> MRPPFTYATLIRWAILEAPEKQRTLNEIYHWFTRMFA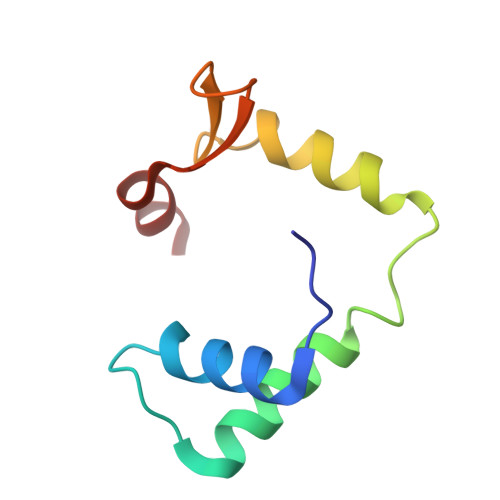FFRNHPATWKNAIRHNLSLHKCFVRVESEKGAVWTVDELEFRKKR> SNVKTENNDHINLKVAGQDGSVVQFKIKRHTPLSKLMKAYCERQGLSMRQIRFRFDGQPINET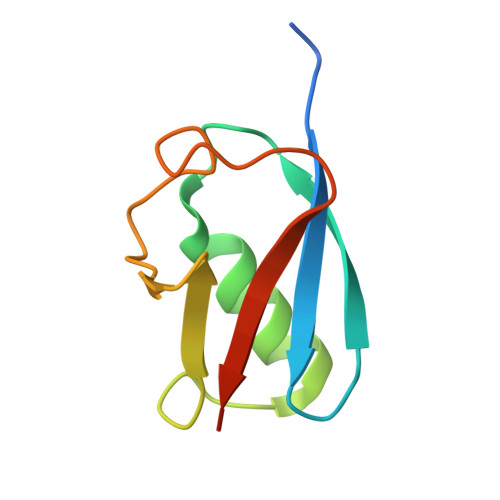DTPAQLEMEDEDTIDVFQQQTGG>MAGLYTTYQLLEVQRKLKTLPAFFLQWFPRQINFQEDMIAFDKVIQDVTRVAPFVAPNVQGRVIK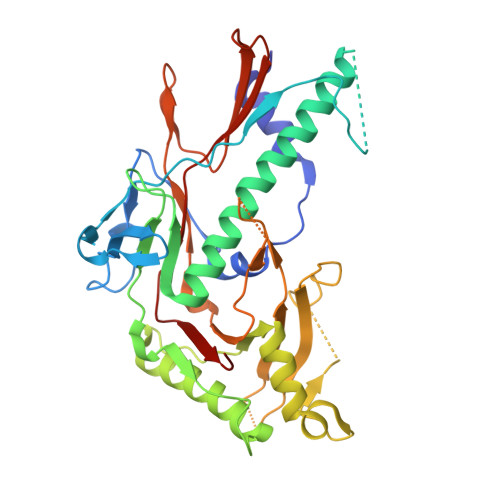ESGYNTKTFKPAYVKPKHVIDPNMIIPRQPGEALGTGTLSIAQRRDRVIAYLLMKHRAMHENTWEWMAAQAAQYGYVDVQGQDYPLVRVDFGRDAALTMTTDWTAAGVTLMDMIADLRDGQRLVSDKSMSGTVIRDYVFGGDAWDQFVKVGGKELWGKDGLMDSTIRGSETNVTRLWDDVEGVQYMGELVGANGAGRMRIWVNTQKYRDQNDQEQFLMKQKAVMGISSAIEGVRCFGAILDKGAGYQALDYFPKMWDQEDPSVEYLMSQGAPLMVPADPNASFLLTVMS[2x]> MDVPGPVSRRAAAAAATVLLRTARVRRECWFLPTALLCAYGFFASLRPSEPFLTPYLLGPDKNLTEREVFNEIYPVWTYSYLVLLFPVFLATDYLRYKPVVLLQGLSLIVTWFMLLYAQGLLAIQFLEFFYGIATATEIAYYSYIYSVVDLGMYQKVTSYCRSATLVGFTVGSVLGQILVSVAGWSLFSLN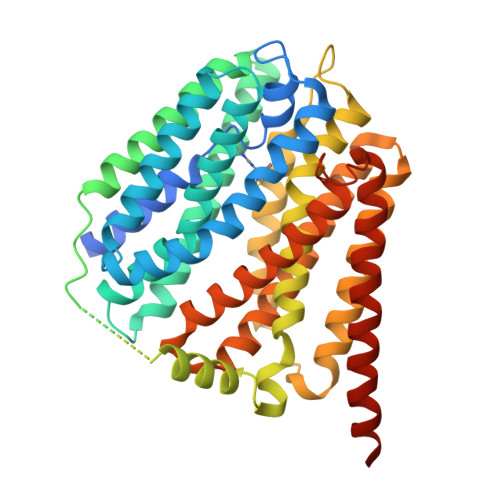VISLTCVSVAFAVAWFLPMPQKSLFFHHIPSTCQRVNGIKVQNGGIVTDTPASNHLPGWEDIESKIPLNMEEPPVEEPEPKPDRLLVLKVLWNDFLMCYSSRPLLCWSVWWALSTCGYFQVVNYTQGLWEKVMPSRYAAIYNGGVEAVSTLLGAVAVFAVGYIKISWSTWGEMTLSLFSLLIAAAVYIMDTVGNIWVCYASYVVFRIIYMLLITIATFQIAANLSMERYALVFGVNTFIALALQTLLTLIVVDASGLGLEITTQFLIYASYFALIAVVFLASGAVSVMKKCRKLEDPQSSSQVTTS> MDPGTVLEISRSLKKRMQDILKKDNANNLEGRPATGKIENVEEISDILMSKALQESLLDEGILDEIKGWLEPLPDKSMPNIKIRKRLLDVLKTMKIHKEHLVTSGVGKIVYFYSINPKESKEVRASAKALVQKWTNEVFKPEGGD;> GSHMREISEESISSIDYGDRDSLFFEIFGT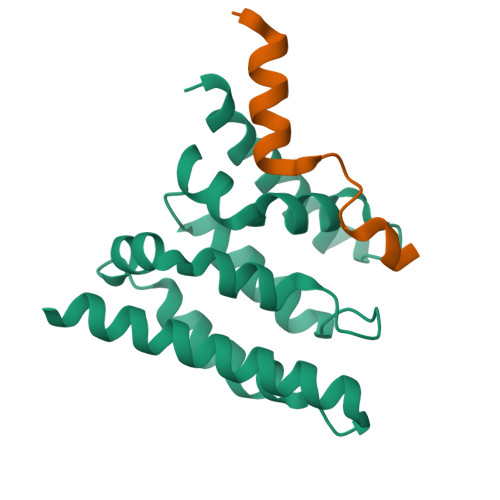GEEYRYVLESDP> LKLTESNRSPRTTNTTDLSGKVAVVTGAAAGLGRAEALGLARLGATVVVNDVASALDASDVVDEIGAAAADAGAKAVAVAGDISQRATADELLASAVGLGGLDIVVNNAGITRDRMLFNMSDEEWDAV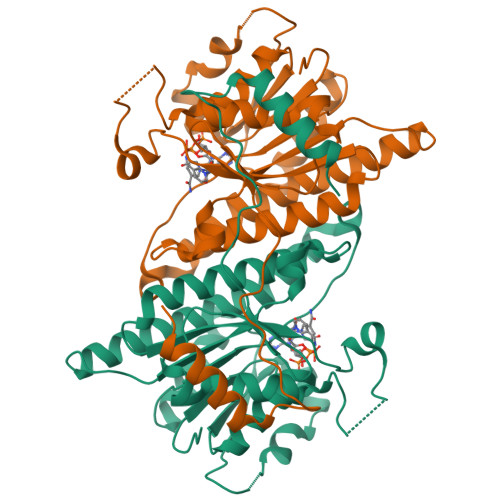IAVHLRGHFLLTRNAAAYWRDKAKDAEGGSVFGRLVNTSSEAGLVGPVGQANYAAAKAGITALTLSAARALGRYGVCANVICPRARTAMTADVFGAAPDVEAGQIDPLSPQHVVSLVQFLASPAAAEVNGQVFIVYGPQVTLVSPPHMERRFSADGTSWDPTELTATLRDYFAGRDPEQSFSATDLMRQ>ASMTGGQQMGRDQAGITGTWYNQLGSTFIVTAGADGALTGTYESAVSANEPDAAEGFRGVRKYVLTGRYDSAPATDGSGTAL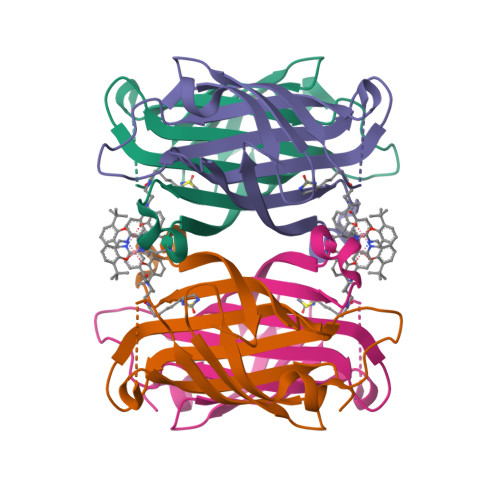GWTVAWKNNYANAHSATTWSGQYVGGAEARINTQWLLTVGTTEANAWHSTLVGHDTFTKVKPSAASIDAAKKAGVNNGNPLDAVQQ[2x]>MGHHHHHHHHHHSSGHIEGRHMKKPRIDMHSHFFPRISEQEAAKFDANHAPWLQVSAKGDTGSIMMGKNNFRPVYQALWDPAFRIEEMDAQGVDVQVTCATPVMFGYTWEANKAAQWAERMNDFALEFAAHNPQRIKVLAQVPLQDLDLACKEASRAVAAGHLGIQIGNHLGDKDLDDATLEAFLTHCANEDIPILVHPWDMMGGQRMKKWMLPWLVAMPAETQLAILSLILSGAFERIPKSLKICFGHGGGSFAFLLGRVDNAWRHRDIVREDCPRPPSEYVDRFFVDSAVFNPGALELLVSVMGEDRVMLGSDYPFPLGEQKIGGLVLSSNLGESAKDKIISGNASKFFNINV[3x]

ACMSD, the enzyme responsible for decarboxylating α-amino-β-carboxymuconate-ε-semialdehyde (ACMS) to produce α-aminomuconate-ε-semialdehyde (2-AMS), plays a crucial role in controlling QUIN levels. This zinc-dependent metalloprotein is situated within the tryptophan-kynurenine pathway, where it competes with a spontaneous chemical reaction that converts ACMS directly to QUIN. With the cavity of ACMSD, a mononuclear Zn2+ ion coordinates with His9, His11, His177, Asp294, and a water molecule (residue numbering based on ACMSD from Pseudomonas fluorescens, pfACMSD). ACMSD functions as a dimer, with residue Arg239∗ from the adjacent subunit being crucial for the decarboxylation reaction.

Instead, we obtained crystals when malonate was present in the refined crystallization condition and successfully solved the crystal structure of malonate-bound ACMSD at a resolution of 2.21 Å. Malonate shares similar structural features with ACMS, possessing two carboxylate groups but with one less carbon atom in between. The additional electron density exhibited in the active site accommodates the malonate molecule well, establishing interactions with surrounding residues, including Arg51, Trp194, His228, and Arg239∗. Binding of malonate induced minimal structural alternations. Comparing this binary complex structure to the wild-type ACMSD structure, the RMSD value is 0.276 Å on 258 Cα in total. However, residues within the active site underwent substantial conformational changes to accommodate malonate. Specifically, as depicted in Figure 3B, the side chain of Trp194 rotated approximately 90° to form an H-bond with the carboxylic group of malonate. Additionally, the sulfur atom of Met198 shifted by 3.9 Å upon malonate binding. To facilitate salt-bridge formation with the ligand, the two conformations of the Arg239∗ side chain in the ligand-free structure merged into a single conformation, and the previously missing electron density corresponding to the guanidinium group of Arg51 became visible. The malonate-bound structure demonstrates that the active site’s two catalytically essential Arg residues act as gatekeepers, preventing the substrate from ligating to the metal ion.> TTTVGLVCKDGVVMATEKRATMGNFIASKAA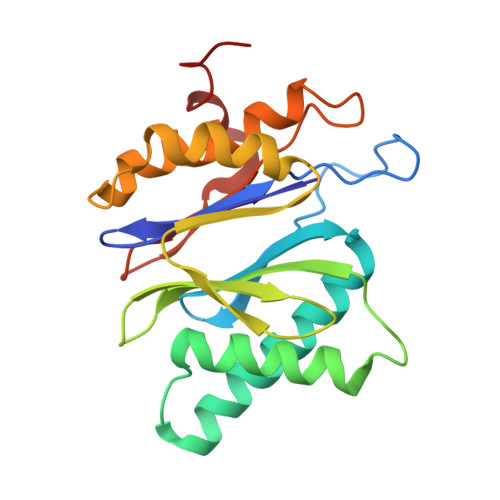KKIYQIADRMAMTTAGSVGDAQFLARIIKIEANLYEIRRERKPTVRAIATLTSNLLNSYRYFPYLVQLLIGGIDSEGKSIYSIDPIGGAIEEKDIVATGSGSLTAYGVLEDRFTPEIGVDEAVELAVRAIYSAMKRDSASGDGIDVVKITEDEFYQYSPEEVEQILAKFRK>[2x]GAGEGQGPKKQTRLGLEAKKEENLADWYSQVITKSEMIEYHDISGCYILRPWAYAIWEAIKDFFDAEIKKLGVENCYFPMFVSQSALEKEKTHVADFAPEVAWVTRSGKTELAEPIAIRPTSETVMYPAYAKWVQSHRDLPIKLNQWCNVVRWEFKHPQPFLRTREFLWQEGHSAFATMEEAAEEVLQILDLYAQVYEELLAIPVVKGRKTEKEKFAGGDYTTTIEAFISASGRAIQGGTSHHLGQNFSKMFEIVFEDPKIPGEKQFAYQNSWGLTTRTIGVMTMVHGDNMGLVLPPRVACVQVVIIPCGITNALSEEDKEALIAKCNDYRRRLLSVNIRVRADLRDNYSPGWKFNHWELKGVPIRLEVGPRDMKSCQFVAVRRDT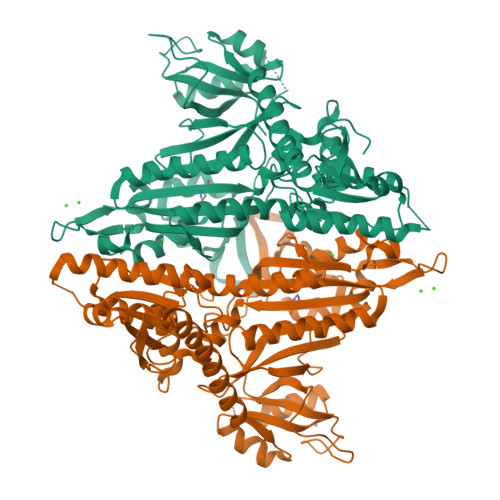GEKLTVAENEAETKLQAILEDIQVTLFTRASEDLKTHMVVANTMEDFQKILDSGKIVQIPFCGEIDCEDWIKKTTARDQDLEPGAPSMGAKSLCIPFKPLCELQPGAKCVCGKNPAKYYTLFGRSY N~2~-{(2R)-2-hydroxy-2-[4-(trifluoromethyl)phenyl]acetyl}-N-[(pyridin-2-yl)methyl]-L-cysteinamide 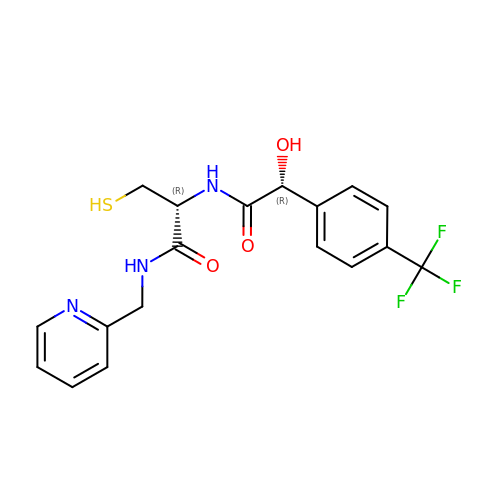| C18 H18 F3 N3 O3 S | MMSMEDXVHMERGZ-LSDHHAIUSA-N> PELPEVETIRRTLLPLIVGKTIEDVRIFWPNIIRHPRDSEAFAARMIGQTVRGLERRGKFLKFLLDRDALISHLRMEGRYAVASALEPLEPHTHVVFCFTDGSELRYRDVRKAGTMHVYAKEEADRRPPLAELGPEPLSPAFSPAVLAERAVKTKRSVKALLLDCTVVAGFGNIYVDESLFRAGILPGRPAASLSSKEIERLHEEMVATIGEAVMKGGSTVRTYVNTQGEAGTFQHHLYVYGRQGNPCKRCGTPIEKTVVAGRGTHYCP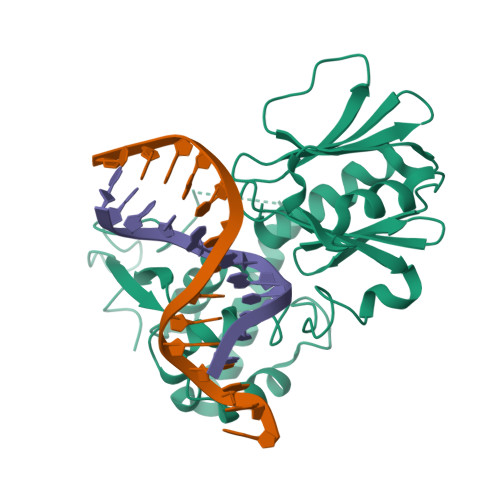RCQR> EKYEGDWVNGKMHGHGKYIYSDGGVYEGDWIDGKMHGKGTYVFPNGNVYEGEWAHDMKDGYGVLTYQNGEKYEGYWKQDKVHGKGTLTYTRGDKYIGDWMDAKKDGEGELIYANGDRFKGQWADDRANGFGVFTYANGNRYEGEWTDDKRHG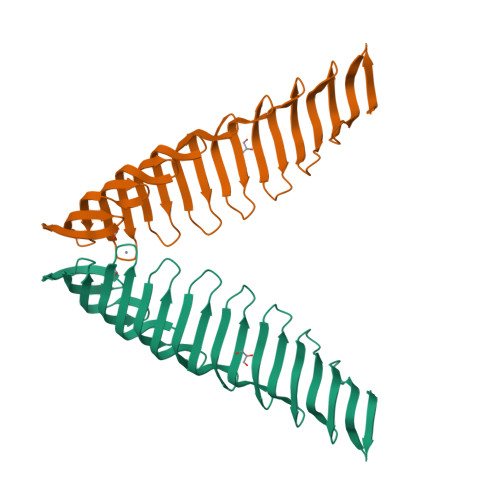RGVFYCAEDGSAYEGEFVGGRKEGNGILRLATGHQLEGTWSGGQLVRVTSFVFAQDSPWLNVDL>[2x]DAYTWKNVRVDGGGFVPGIVFNRKEKNLAYARTDIGGAYRWDQSGKRWVPLLDSLDWDHWGWTGVVSLASDSVDPNKVYVAAGTYTNSWDPGNGAILRSSNRGASWQSTTLPFKLGGNMPGRGMGERLAVDPNRNSVLYLGAPSGNGLWRSTDSGMTWSKVTSFPNPGTYVQDASDTSGYLSDNQGVVWVTFDERTGSSGSATKTIYVGVADKDNTVYRSTDAGVTWSRVAGQPTGYLSHKGVLDAKDGYLYLTTSDKGGPYDGEKGQVWRYTTATGEWKNISPMADADTYFGYSGLTVDRQKPGTLMVTGYSSWWPDTQIFRSTDSGATWTRAWDFTSYPNRSLRYTQDVSSVPWLTFGTNPTPPEVTPKLGWMTEALEIDPFDSNRMMYGTGATVYGTENLGNWDTGGKIAITPMIRGLEETAVNDLASPPTGAPLLSALGDIGGFRHTDLDAVPARMYTSPTFTTTTSLDYAETNPN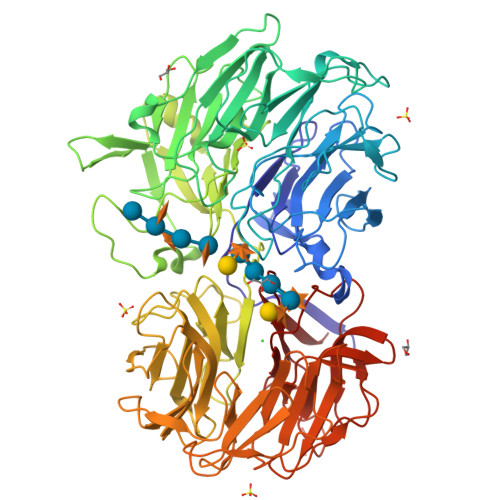TVVRVGNNDSAPRIAFSTDNGANWFQGSEPSGVTGGGTVAAAADGSGFVWAPEGSSAVYHTTGFGNSWSVSSGIPAGAVVESDRKNPKKFYGFKAGTFYVSTDGGATFTARASSGLPADGPARFKALPGAEGDIWLAGGSTGGAYGLWHSTDSGATFTKLSGVQQADTIGFGKAAPGASYQTLYTSAKIGGVRGVFRSTDAGASWTRINDDAHQWGWTGASITGDPRVYGRVYVATNGRGILRGDIS>SMGKTLRFEIVSGVNKGYFHTNSQSESLDLVGGIWQKIA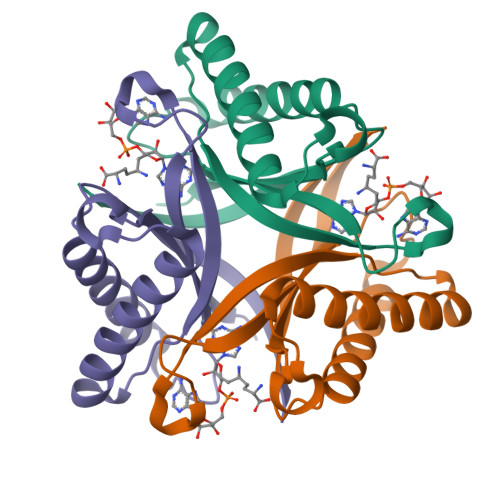KEEFEKSNIYVSAVIKPSKTVYNQEWGCPENGEETVVLTGVANEEFVDDIEKWKDTVIKLAKELKNQMKQSTLTCEFIETELHYFK[3x]>[2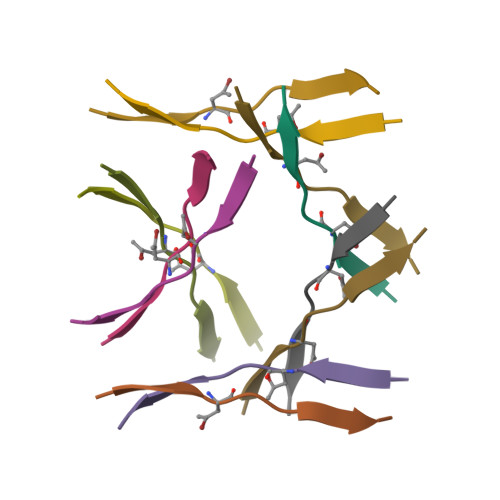x]KVKVXWDVIEV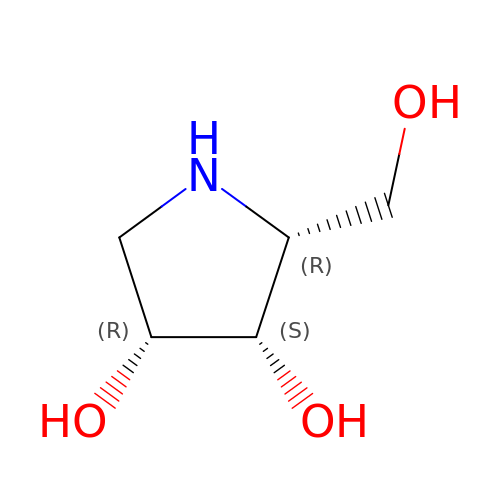DIDEOXY-IMINO-LYXITOL | C5 H11 N O3 | OQEBIHBLFRADNM-WDCZJNDASA-N> GG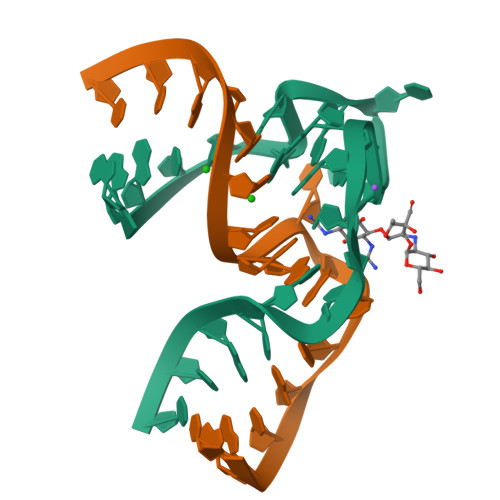AUCGCAUUUGGACUUCUGCC;> CGGCACCACGGUCGGAUC PHENYL-5-(1H-PYRAZOL-3-YL)-1,3-THIAZOLE 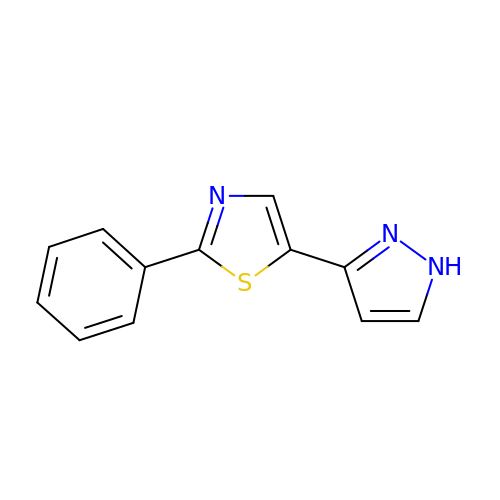| C12 H9 N3 S | NRAHRUHGPGBWSI-UHFFFAOYSA-N> MGSSHHHHHHENLQFQGGGNRGMSRNQDAYAEKMDMTLDALNFLLGVEHLASAFYVQAVNNFTADDFKAAGLAQRDYDQFVGVRNNEVDHRDTLISVIKSLGGKPNPPCKYTFPVTDVASVLKVSRTLENADKPAYLGALRDIKSVELRTSVQGALSGDSAHAAFFAYLTGKAPAPGPVDGPLTQRHIATLAQDFIVSCPYPAPKPFPKLTLSPQSGPVGTVVATTCAQDVDTNGVMCAIISGNQGTLMQRPGQAKDGSGAATCTIPPGVKGILFIAWVRGRDVLNVGVDDSSTVCGPNYFLLSALGDAVPGV

Here, we focused on the tardigrade Ramazzottius varieornatus, one of the toughest animals on Earth. A transcriptome database of R. varieornatus shows that genes encoding a Ferritin‐like protein are upregulated during desiccation or ultraviolet radiation. This protein shows sequence similarity to enigmatic proteins in desiccation‐tolerant bacteria and plants, which are hypothesized to be desiccation‐related. Our results indicate that through cleaning up damaged metabolites or regulation of metabolite levels, this phosphatase family can contribute to stress tolerances.

We determined an atomic (1.05 Å) resolution crystal structure of a Ferritin‐like protein from R. varieornatus. The structure revealed a dinuclear metal binding site, and we showed that this Ferritin‐like protein has phosphatase activity toward several metabolite compounds including unusual nucleotide phosphates produced by oxidative or radiation damage.>MATKENTENVLRSYLAKYKKTLIIVGLFSLFINILFLLPSIYMLAVYDIVVPSTSVPTLLVITALAVVLYFALGLLQSVRAKVMQIISLKLDSELNKEVFTSSFEYAIRNPSKASAQPINDLYQLKQFLTSPVLFAIFDLPWVPIYFGVLFVFHVYYGVMAILSMAVIVALAILNEYITKKKLKESNELLVRSTNFLNRALLNAEVVEALGMRNNLYKKWMNFYSKHLSAFEEATDRNNFLSNLTRIFRIMAQSLMLGLGGYLAIKHEITTGMIVAGSILLGRILGPIDTIVNGWRQIGNTKVAYTRLNEFLKFLRFKREVSVKLPEPKGEIELSNVVVVPPEGKTPVLRNINMRILPGEFVAIIGPSGSGKSSLVRTILGIWLPVHGTVEIDGADLKQWDRDYFGKFVGYLPQDIELFEGTVAENIARFGELDSEKIIEAAKLSGAHDVIIKLPDGYDTYIGPGGITLSGGQRQRIALARALYGNPRIVILDEPDSNLDEQGEQALYNALIELKKRKVTTIIVSHRIRLLNLVDKIAIMQDGTLKAFGKADIIIQKLLRKNVNLEHHHHH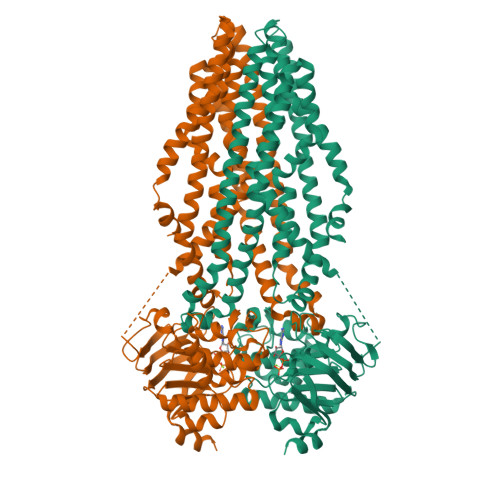H[2x]> MTAPILLLDGASMWFRSYFGVPSSIKAPDGRPVNAVRGFI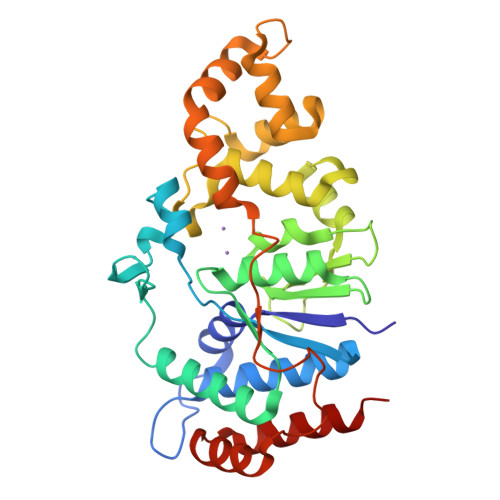DAISTLVTREKPRRLVVCRDDDWRPQWRVDLIPSYKAHRVAEPEPDGVPDIEEVPDDLTPQVNMILELLDAFGIPTAGAAGFEADDVLGTLSAREERDPVVVVSGDRDLLQLVRDEPAPQVRVLYLGRGLAKATKWGPAEVAEQYGVPLDRAGTAYAELALLRGDPSDGLPGVAGIGEKTAASLLAKHGSLQNILDAAHDPKSGLSKAHRTKLLGAVDYIAAAETVVRVATDAPVTFSTPTDTLPLAAGDPARVAELAAAYGVSSSISRLQTALDQLPD>MSTNITFHASALTRSERTELRNQRGLTIWLTGLSASGKSTLAVELEHQLVRDRRVHAYRLDGDNIRFGLNKDLGFSEADRNENIRRIAEVAKLFADSNSIAITSFISPYRKDRDTARQLHE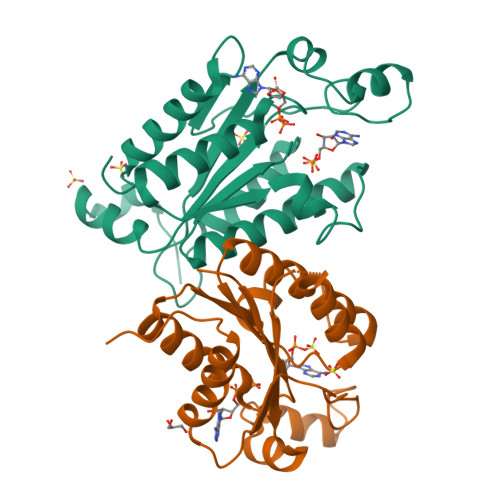VATPGEETGLPFVEVYVDVPVEVAEQRDPKGLYKKAREGVIKEFTGISAPYEAPANPEVHVKNYELPVQDAVKQIIDYLDTKGYLPAKKE[4x]>QCTVRYNVADCSHLKLTHIPDDLPSNITVLNLTHNQLRRLPPTNFTRYSQLAILDAGFNSISKLEPELCQILPLLKVLNLQHNELSQISDQTFVFCTNLTELDLMSNSIHKIKSNPFKNQKNLIKLDLSHNGLSSTKLGTGVQLENLQELLLAKNKILALRSEELEFLGNSSLRKLDLSSNPLKEFSPGCFQTIGKLFALLLNNAQLNPHLTEKLCWELSNTSIQNLSLANNQLLATSESTFSGLKWTNLTQLDLSYNNLHDVGNGSFSYLPSLRYLSLEYNNIQRLSPRSFYGLSNLRYLSLKRAFTKQSVSLASHPNIDDFSFQWLKYLEYLNMDDNNIPSTKSNTFTGLVSLKYLSLSKTFTSLQTLTNETFVSLAHSPLLTLNLTKNHISKIANGTFSWLGQLRILDLGLNEIEQKLSGQEWRGLRNIFEIYLSYNKYLQLSTSSFALVPSLQRLMLRRVALKNVDISPSPFRPLRNLTILDLSNNNIANINEDLLEGLENLEILDFQHNNLARLWKRANPGGPVNFLKGLSHLHILNL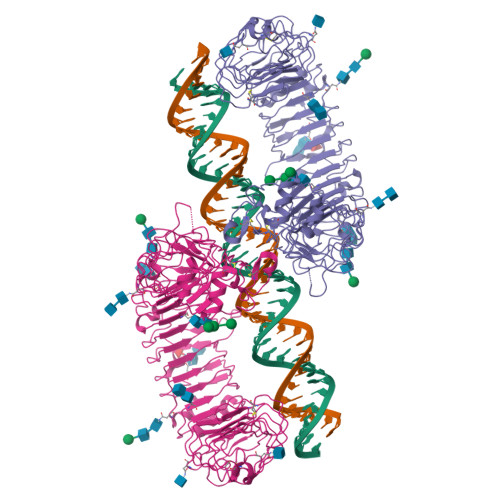ESNGLDEIPVGVFKNLFELKSINLGLNNLNKLEPFIFDDQTSLRSLNLQKNLITSVEKDVFGPPFQNLNSLDMRFNPFDCTCESISWFVNWINQTHTNISELSTHYLCNTPHHYYGFPLKLFDTSSCKDSAPFENLYFQGHHHHHHWSHPQFEK[2x]> MYVCLCQGVTDNQIRDAIYEGCCSYEEVREATGVGTQCGKCAS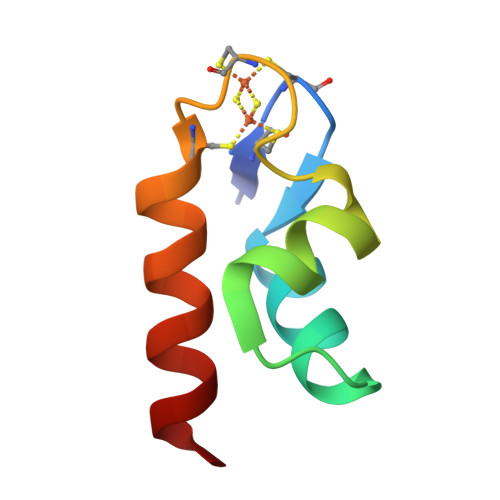LAKQVVRETLNDL> DATNYNHVFASRFAAFNELLSI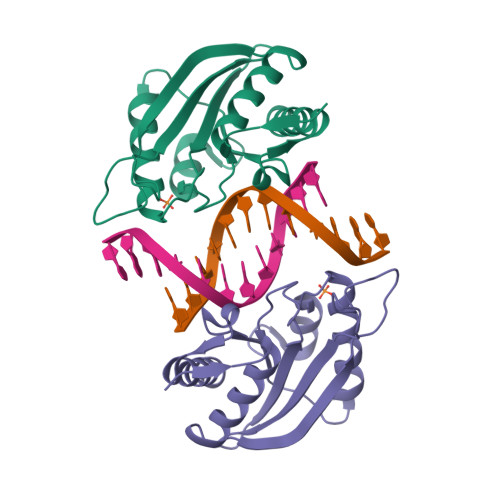LKTKFRCRVIFEETLVLPKVGRSRLHLCKDGSPRVIKAVGVWRNASEFILLEVDASDGVKMLSTKVLIGVNRETWQSDFERIRRGIVRNSLNWPNGLLYQLYGKEGNRGVNHPKGLSELEVSREDMEGWGERLIRELEHHHHHH>[2x]GGGGTGGG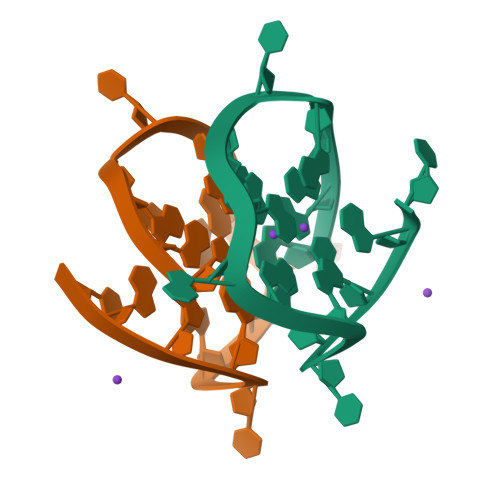GGGTGGGT> NYKKPKLLYCSNGGHFLRILPDGTVDGTRDRSDQHIQLQLSAESVGEVYIKSTETGQYLAMDTDGLLYGSQTPNEECLFLERLEENHYNTYISKKHAEKNWFVGLKKNGSC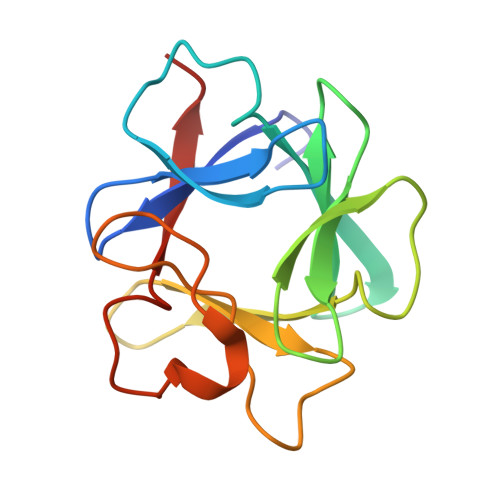KRGPRTHYGQKAILFLPLPVSSD>[2x]MMRRTLENRNAQTKQLQTAVSNVEKHFGELC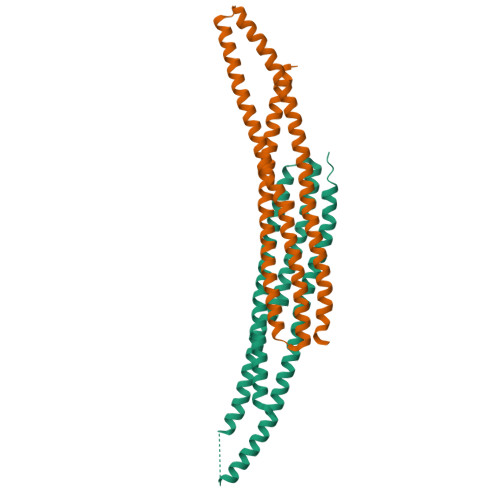QIFAAYVRKTARLRDKADLLVNEINAYAATETPHLKLGLMNFADEFAKLQDYRQAEVERLEAKVVEPLKTYGTIVKMKRDDLKATLTARNREAKQLTQLERTRQRNPSDRHVISQAETELQRAAMDASRTSRHLEETINNFERQKMKDIKTIFSEFITIEMLFHGKALEVYTAAYQNIQNIDEDEDLE>MLLEAIFHEAKGSYAYPISETQLRVRLRAKKGDVVRCEVLYADRYASPEEELAHALAGKAGSDERFDYFEALLECSTKRVKYVFLLTGPQGEAVYFGETGFSAERSKAGVFQYAYIHRSEVFTTPEWAKEAVIYQIFPERFANGDPSNDPPGTEQWAKDARPRHDSFYGGDLKGVIDRLPYLEELGVTALYFTPIFASPSHHKYDTADYLAIDPQFGDLPTFRRLVDEAHRRGIKIILDAVFNHAGDQFFAFRDVLQKGEQSRYKDWFFIEDFPVSKTSRTNYETYAVQVPAMPKLRTENPEVKEYLFDVARFWMEQGIDGW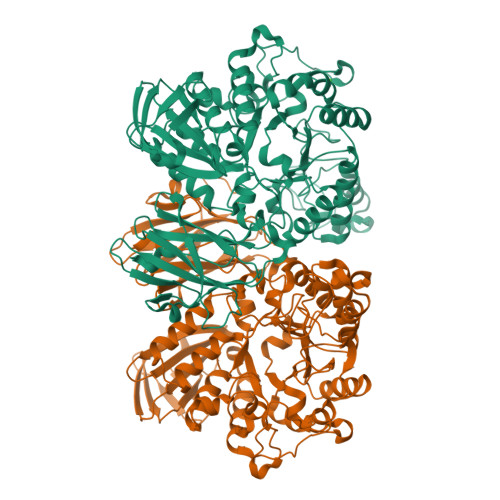RLDVANEVDHAFWREFRRLVKSLNPDALIVGEIWHDASGWLMGDQFDSVMNYLFRESVIRFFATGEIHAERFDAELTRARMLYPEQAAQGLWNLLDSHDTERFLTSCGGNEAKFRLAVLFQMTYLGTPLIYYGDEIGMAGATDPDCRRPMIWEEKEQNRGLFEFYKELIRLRHRLASLTRGNVRSWHADKQANLYAFVRTVQDQHVGVVLNNRGEKQTVLLQVPESGGKTWLDCLTGEEVHGKQGQLKLTLRPYQGMILWNGR[2x]>[2x]GGCUUGG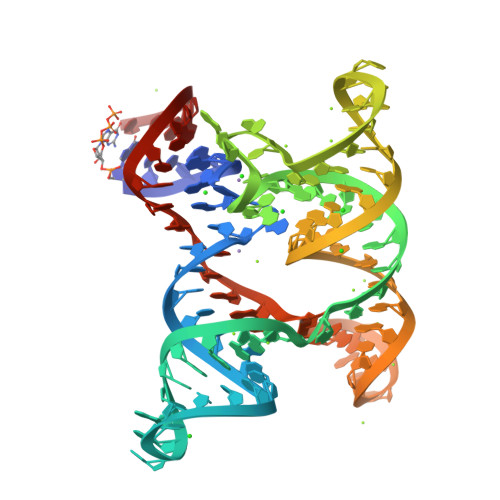GGAGUAGCCUGCUUUCGGAAACGAAAGCGCCUGUAUCAACAUACUCGGCGAAAGCCGUGGUGCAGGACCGAAAGGUCUGGCGAGACCAGGCC> MAATNMTDNVTLNNDKISGQAWQAMRDIGMSRFELFNGRTQKAEQLAAQAEKLLNDDSTDWNLYVKSDKKAPVEGDHYIRINSSITVAEDYLPAGQKNDAINKANQKMKEGDKKGTIEALKLAGVSVIENQELIPLQQTRKDVTTALSLMNEGKYYQA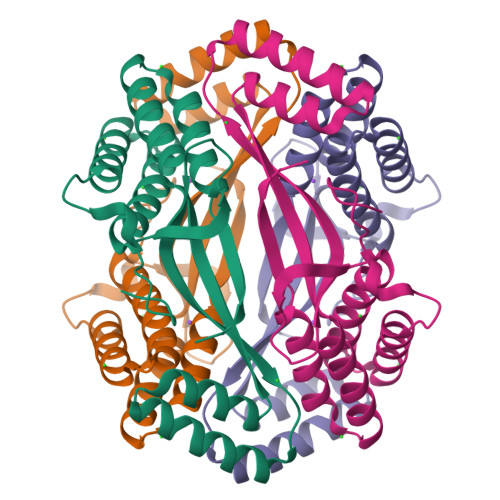GLLLKSAQDGIVVDSQSVQLEHHHHHH>[7x]GAMDMQAKVENPLKSLRTAI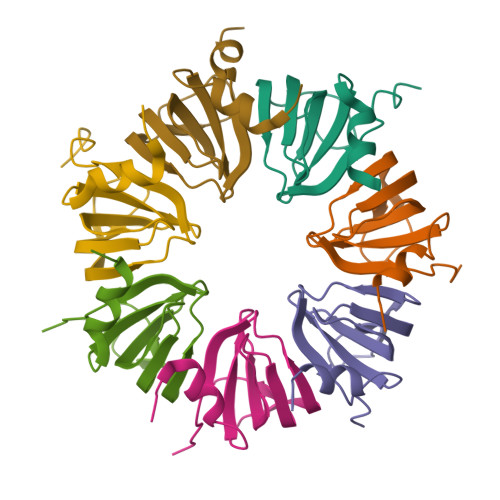NRIVLVKLKDGSEYIGKLEQTDGTMNLVLRDCTEIREGTSEPVAKYGRVLIRGSNILFISVDYETVMNSEK> GSHMGTLEKKLDNLVNTILLKAENQHELLFGACQSDVKLTNTQEHILMLLSQQRLTNTDLAKALNISQAAVTKAIKSL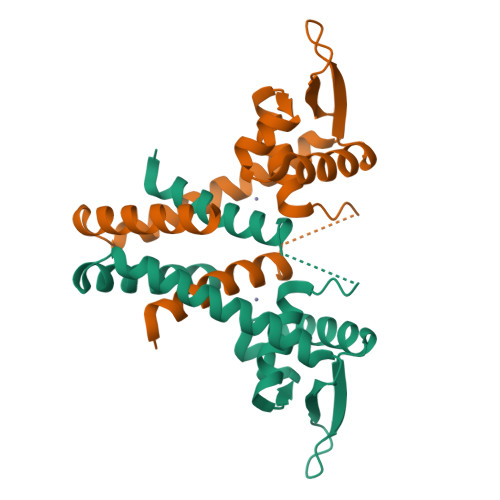VKQDMLAGTKDTVDARVTYFELTELAKPIASEHTHHHDETLNVYNRLLQKFSAKELEIVDKFVTVFAEELEG>MNKKSKQQEKLYNFIIAKSFQQPVGSTFTYGELRKKYNVVCSTNDQREVGRRFAYWIKYTPGLP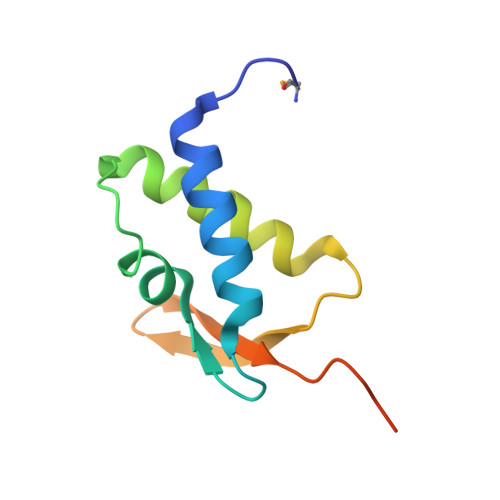FKIVGTKNGSLLYQKIGINPCNNSTPSKGGDC[2x]>GARGGSDLEIDNEGVIEADTDAPQEMGDENAEITEAMMDEANEKKGAAIDALNDGELQKAIDLFTDAIKLNPRLAILYAKRASVFVKLQKPNAAIRDCDRAIEINPDSAQPYKWRGKAHRLLGHWEEAARDLALAC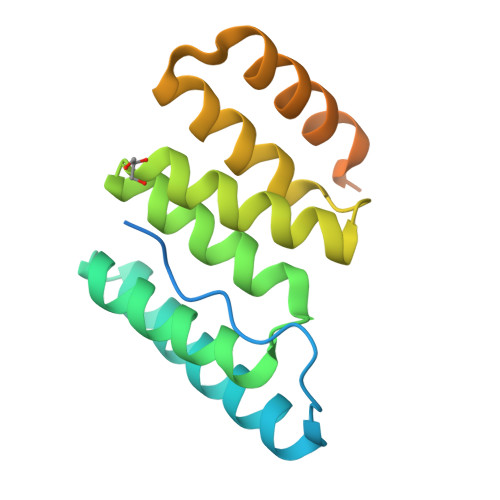KLDYDEDASAMLREVQPRAQKIAEHRRKYERKREEREIK[2x]> PVQLNLLYVQARDDILNGSHPVSFDKACEFAGYQCQIQFGPHNEQKHKPGFLELKDFLPKEYIKQKGERKIFMAHKNCGNMSEIEAKVRYVKLARSLKTYGVSFFLVKEKMKGKNKLVPRLLGITKECVMRVDEKTKEVIQEWSLT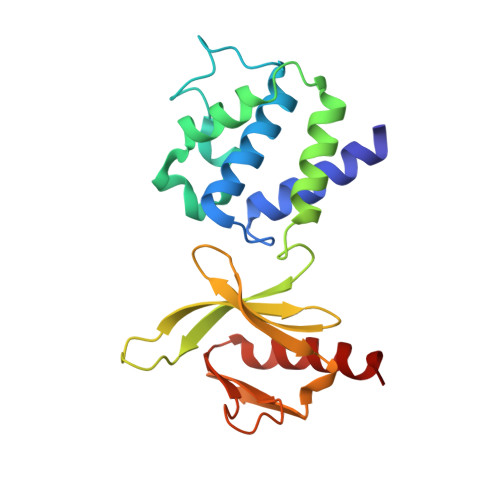NIKRWAASPKSFTLDFGDYQDGYYSVQTTEGEQIAQLIAGYIDIIL>[2x]MVLYFIGLGLYDERDITVKGLEIAKKCDYVFAEFYTSLMAGTTLGRIQKLIGKEIRVLSREDVELN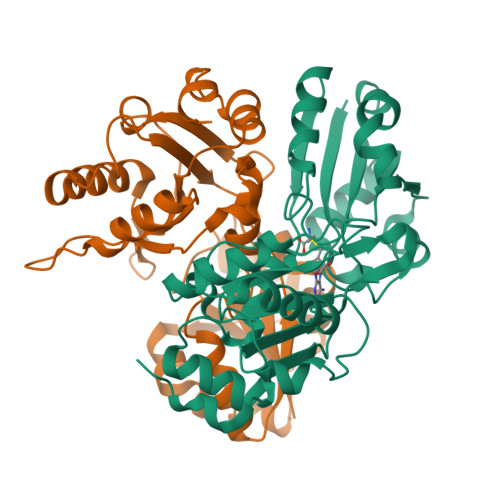FENIVLPLAKENDVAFLTPGDPLVATTHAELRIRAKRAGVESYVIHAPSIYSAVGITGMHIYKFGKSATVAYPEGNWFPTSYYDVIKENAERGLHTLLFLDIKAEKRMYMTANEAMELLLKVEDMKKGGVFTDDTLVVVLARAGSLNPTIRAGYVKDLIREDFGDPPHILIVPGKLHIVEAEYLVEIAGAPREILRVNV(3S)-3-(benzotriazol-2-yl)piperidine-2,6-dione | C11 H10 N4 O2 | 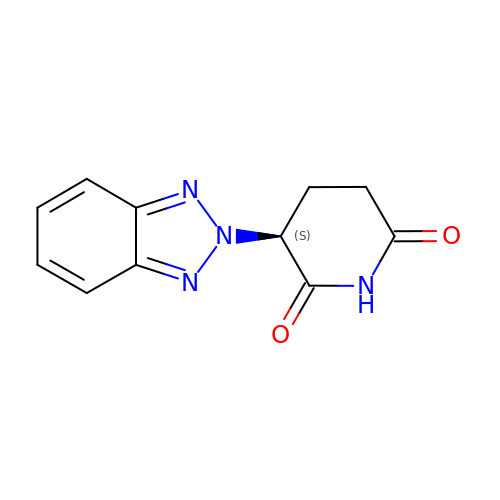QFGWCBAWFMYBCK-VIFPVBQESA-N> PTHIAICLYYKLGETPLPLVIETGKDAKALQIIKLAELYDIPVIEDIPLATSLYKNIHKGQYITEDFFEPVAQLIRIAIDL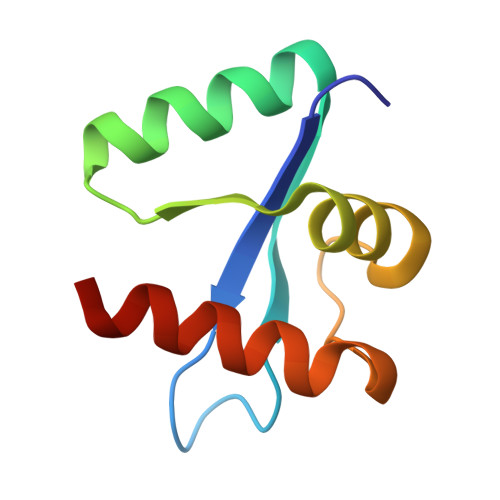DY> MAKNRRDRNSWGGFSEKTYEWSSEEEEPVKKAGPVQVLIVKDDHSFELDETALNRILLSEAVRDKEVVAVSVAGAFRKGKSFLMDFMLRYMYNQESVDWVGDYNEPLTGFSWRGGSERETTGIQIWSEIFLINKPDGKKVAVLLMDTQGTFDSQSTLRDSATVFALSTMISSIQVYNLSQ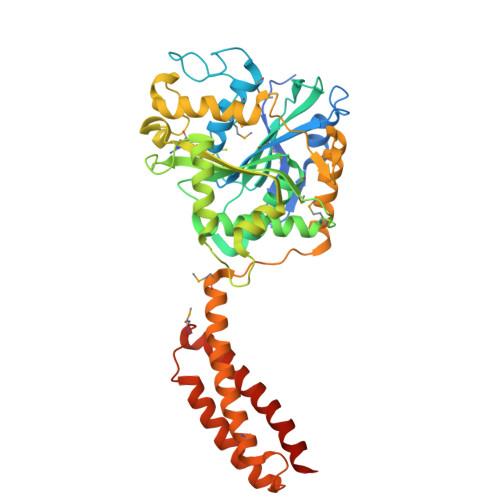NVQEDDLQHLQLFTEYGRLAMEETFLKPFQSLIFLVRDWSFPYEFSYGADGGAKFLEKRLKVSGNQHEELQNVRKHIHSCFTNISCFLLPHPGLKVATNPNFDGKLKEIDDEFIKNLKILIPWLLSPESLDIKEINGNKITCRGLVEYFKAYIKIYQGEELPHPKSMLQATAEANNLAAVATAKDTYNKKMEEICGGDKPFLAPNDLQTKHLQLKEESVKLFRGVKKMGGEEFSRRYLQQLESEIDELYIQYIKHNDSKNIFHAART> GPHMTRHPLQNRWALWYLKADRNKEWEDCLKMVSLFDTVEDFWSLYNHIQSAGGLNWGSDYYLFKEGIKPMWEDVNNVQGGRWLVVVDKQKLQRRTQLLDHYWLELLMAIVGEQFDEYGDYICGAVVNVRQKGDKVSLWTRDATRDDVNLRIGQVLKQKLSIPDTEILRYEVHKDSSARTSSTVKPRICL;> GPHMIRYNRDTLMTARDTKRAPIPDE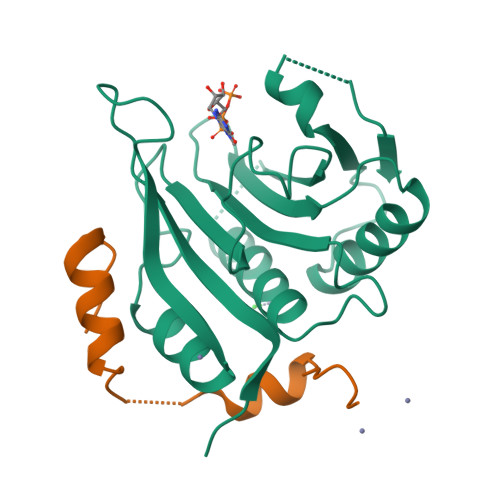MLQEINRVAPDILIA>[4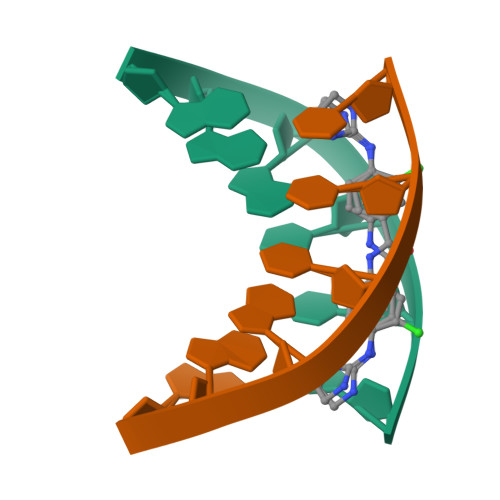x]AAATTT>[4x]QQFPQFHVKSGLQIKKNAIIDDYKVTSQVLGLGINGKVLQIFNKRTQEKFALKMLQDCPKARREVELHWRASQCPHIVRIVDVYENLYAGRKCLLIVMECLDGG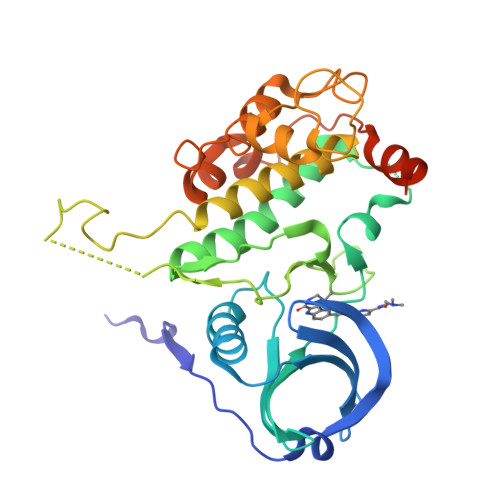ELFSRIQDRGDQAFTEREASEIMKSIGEAIQYLHSINIAHRDVKPENLLYTSKRPNAILKLTDFGFAKETTSHNSLTTPCYTPYYVAPEVLGPEKYDKSCDMWSLGVIMYILLCGYPPFYSNHGLAISPGMKTRIRMGQYEFPNPEWSEVSEEVKMLIRNLLKTEPTQRMTITEFMNHPWIMQSTKVPQTPLHTSRVLKEDKERWEDVKEEMTSALATMR> MDPPVTHDLRVSLEEIYSGCTKKMKISHKRLNPDGKSIRNEDKILTIEVKKGWKEGTKITFPKEGDQTSNNIPADIVFVLKDKPHNIFKRDGSDVIYPARISLREALCGCTVNVPTLDGRTIPVVFKDVIRPGMRRKVPGEGLPLPKTPEKRGDLIIEFEVIFPERIPQT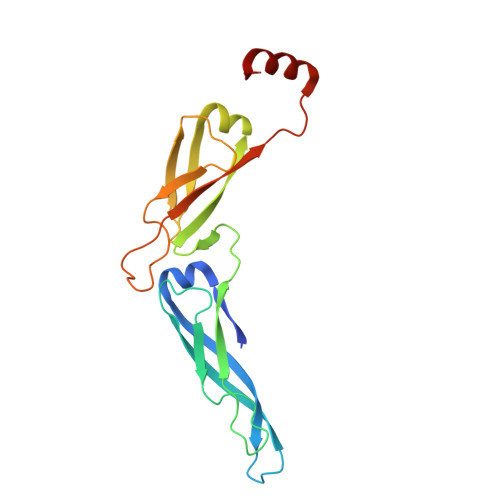SRTVLEQVLPI>AQPTNFHDQLKFAWLAGFVDADGCINAQIVSREDYLLKYQVRVSLTVFQST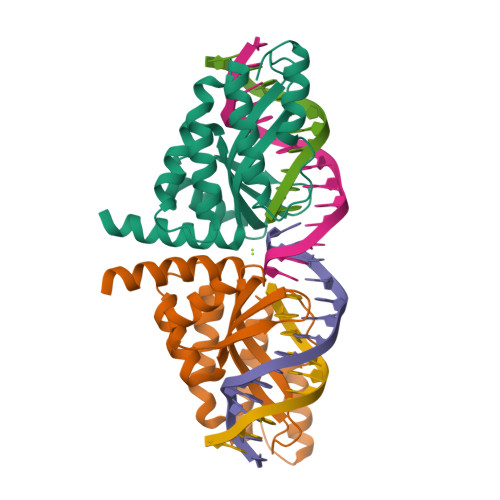TQHFILLDIQKILGCGTVRKRNDGMSEFCVVGGTSLQTTLEKLLPYLQLKRAQAKLVLQIIKKLPNTKDPSVLMEAALLADKVGLLTDGKKRTILAENVRECLKKLGHVVSAALEHHHHHH[2x]> ATPAGSHMRLSELASYVSGKLIGEDKEIKVGIF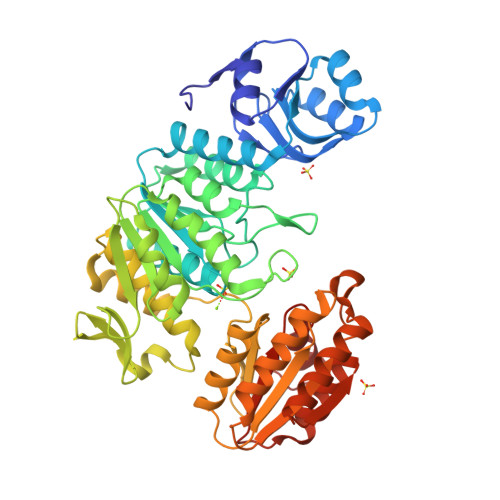NTLGDANPNDIVIRHWIDEKGVEIAKNKEVSALITQNPKGNSLEYAKKLKVPIILVNKIELASAFAIKWTIKNFAPNTYRVVITGTNGKSTTTHMIYHILTHAGKKAFTNTDAKSEFNTLIDPMVAKLLAEKAKKENLEYLVIEVSEVQGWLDRLMKDHAYLMTKSINPNVVVVTNVALDHIGLVNSIEEVFEETSGAVKALEKGFAVLNYDNEFTRKMAKLTNKNVKVFFYGKNCPVTFKSGGIYVNNDLFIKKEELPFKSEYFIQNTLAAISACLCLNIPPDIIKKGILTYKPLKRRFSILCKKPLIIDDFAHNPDGIKMAIKSAKKLTKNKLWVVCAIRGSRGKIINKLNAESLSKTLKNIENYEVVITNSDDVVDNLNKVKKEEEKTFLKTLEKYNINYRFHKKLKTALEETLTNCKKDDTILLIGAQGMDPASKLLKKIKVIPCS>MQKMLYFDDDVKQIVDHMFFKGFMFNDERIDRYFKESFTLRFLYREIGRQTVESFASQVLYITMTHEDYIYRVYGSDMYKYIEQVTDTQSQDLGKAIENAIEQGQTKDRQQDKGHEEYKDYEDTITKSFDDNRTAESTLPQSKVNIDVDNTVLDYADTNTISRDKNTSETVSEKTGTKDNTFDSLRNGESDTKRNTQSQNEMNRTGLTKQYLIDNLQKLYSMRDTIFKTYDKECFLHIW[2x];> MADRKLTHFKFFYNTPLTDYQNTIHFSSNNERDNYFLNENHFNAIDYKNIPFNFIRDRNMVN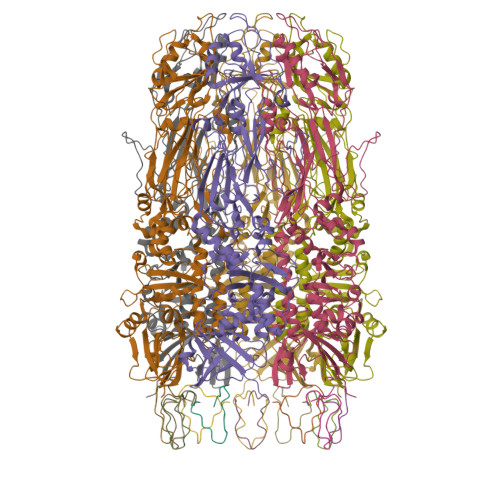LEQMSWQDAQGINYCTFKSDFENRRYYAFVNQIEYVNDHVTRMYLVIDTVMTYTQGNVLSTVQNAFVERQHLPRDVYNYLLPSLRNNDDVIKASNKYYLNNYLEQFGGNLVLFQSSADLSKKFGTKKEPNLESSKGITYDYITSPVNLYVMNREDFNNFMDKMSKYPWITQNFQKIILIPATFINKDDLEAVKTQEDIKGLMTLKNDKLSNEWELKELRVPFERLQYMLNSNQDELKHLVRNEYLTIEIYSWNGDSLLLDAGKITERTGVKLKTKSIIGYHNEVRIYPVDYNSAPNEKPIKASDNSILIDTGSFLNTAITFDSFAEVPILIDNGLLAQSQQANKQKNAQSNLISNRINNVVNGNDLKSRFYDAVSIGSNLSPTALFSKFNDEYNYYKELRAEYKDLALQPPTVTSSQMGNAFQIANSINGLTMKIGVPAPFDMDNIQRYYFMLGFETNDQAGTPFPIDSWTVCNYLRMRGTYTIDGIDPMLLEQLKVLLETGVRFWHNDGTNNPMAQNVFKNKFRK> R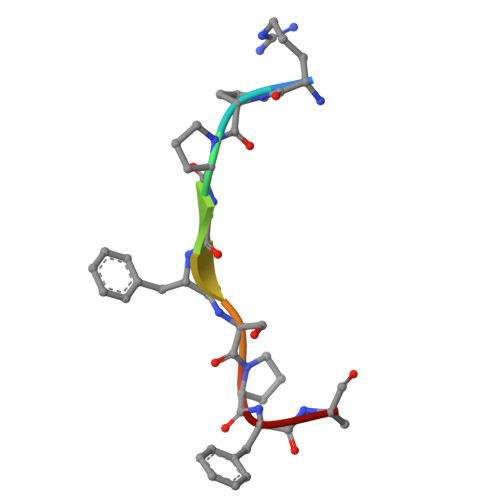PPGFSPFA>AATYAQTLQNIPETNVTTLDNGLRVASEESSQPTCTVGVWIGAGSRYENEKNNGAGYFVEHLAFKGTKKRPCAAFEKEVESMGAHFNGYTSREQTAFYIKALSKDMPKVVELLADVVQNCALEESQIEKERGVILQELKEMDNDMTNVTFDYLHATAFQGTALARTVEGTTENIKHLTRADLASYIDTHFKAPRMVLAAAGGISHKELVDAARQHFSGVSFTYKEDAVPILPRCRFTGSEIRARDDALPVAHVALAVEGPGWADPDNVVLHVANAIIGRYDRTFGGGKHLSSRLAALAVEHKLCHSFQTFNTSYSDTGLFGFHFVADPLSIDDMMFCAQGEWMRLCTSTTESEVKRAKNHLRSAMVAQLDGTTPVCETIGSHLLNYGRRISLEEWDSRISAVDARMVRDVCSKYIYDKCPALAAVGPIEQLLDYNRIRSGMYWIRF[2x];>[2x]SLKVAPKVAVSAAAERVKLCPGAEDLEITKLPNGLIIASLENFSPASRIGVFIKAGSRYETTANLGTAHLLRLASPLTTKGASSFRITRGIEAVGGSLSVYSTREKMTYCVECLRDHVDTVMEYLLNVTTAPEFRPWEVTDLQPQLKVDKAVAFQSPQVGVLENLHAAAYKTALANPLYCPDYRIGKITSEQLHHFVQNNFTSARMALVGIGVKHSDLKQVAEQFLNIRSGAGTSSAKATYWGGEIREQNGHSLVHAAVVTEGAAVGSAEANAFSVLQHVLGAGPLIKRGSSVTSKLYQGVAKATTQPFDASAFNVNYSDSGLFGFYTISQAAHAGEVIRAAMNQLKAAAQGGVTEEDVTKAKNQLKATYLMSVET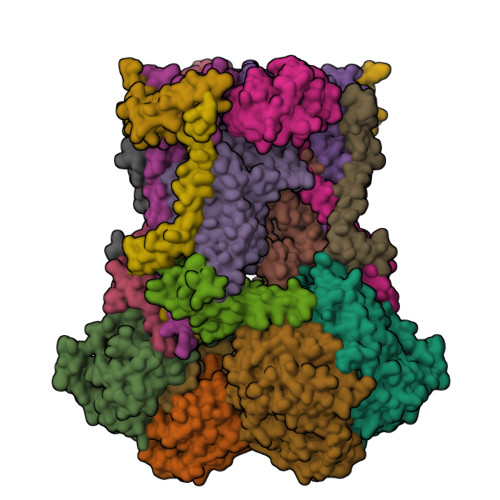AQGLLNEIGSEALLSGTHTAPSVVAQKIDSVTSADVVNAAKKFVSGKKSMAASGDLGSTPFLDEL;>[2x]MAPNIRKSHPLLKMINNSLIDLPAPSNISAWWNFGSLLAVCLMTQILTGLLLAMHYTADTSLAFSSVAHTCRNVQYGWLIRNLHANGASFFFICIFLHIGRGLYYGSYLYKETWNTGVILLLTLMATAFVGYVLPWGQMSFWGATVITNLFSAIPYIGHTLVEWAWGGFSVDNPTLTRFFALHFLLPFAIAGITIIHLTFLHESGSNNPLGISSDSDKIPFHPYYSFKDILGLTLMLTPFLTLALFSPNLLGDPENFTPANPLVTPPHIKPEWYFLFAYAILRSIPNKLGGVLALAASVLILFLIPFLHKSKQRTMTFRPLSQTLFWLLVANLLILTWIGSQPVEHPFIIIGQMASLSYFTILLILFPTIGTLENKMLNY;>GELELHPPAFPWSHGGPLSALDHSSVRRGFQVYKQVCSACHSMDYVAFRNLIGVTHTEAEAKALAEEVEVQDGPDENGELFMRPGKISDYFPKPYPNPEAARAANNGALPPDLSYIVNARHGGEDYVFSLLTGYCDPPAGVVVREGLHYNPYFPGQAIGMAPPIYNEILEYDDGTPATMSQIAKDVCTFLRWAAEPEHDQRKRMGLKMLLISALLTSLLYYMKRHKWSVLKSRKMAYRPPK[2x];>VHNDVTVPDFSAYRREDVMDATTSSQTSSEDRKGFSYLVTATACVATAYAAKNVVTQFISSLSASADVLALSKIEIKLSDIPEGKNVAFKWRGKPLFVRHRTQAEINQEAEVDVSKLRDPQHDLDRVKKPEWVILVGVCTHLGCVPIANSGDFGGYYCPCHGSHYDASGRIRKGPAPYNLEVPTYQFVGDDLVVVG[2x];>AARATVAGGGRLMDRIRKWYYNAAGFNKYGLMRDDTLYEDDDVKEALKRLPEDLYNERMFRIKRALDLSLKHRILPKEQWVKYEEDKPYLEPYLKEVIRERLEREAWNKK[2x];>[2x]GIHFGNLARVRHIITYSLSPFEQRAIPNIFSDALPNVWRRFSSQVFKVAPPFLGAYLLYSWGTQEFERLKRKNPADYENDQ;>LRGSGEEEEEELVDPLTTIREHCEQTEKCVKARERLELCDARVSSRSHTEEQCTEELFDFLHARDHCVAHKLFNKLK[2x];>MLSVAARSGPFAPYLSAAAHAVPGPLKAXXXXXXXXXXXXXXLKRPLLCRESMSGRSARRDLVAGISLNAPASVRY[2x];>ALLRQAYSALFRRTSTFALTVVLGAVLFERAFDQGADAIFEHLNEGKLWKHIKHKYEASEE[2x]>GAGAGAGAGEFMKMSGFSIEEK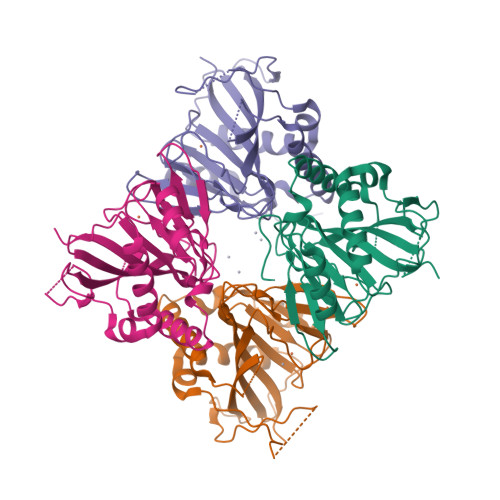VHEFESKGFLEISNEIFLQEEENHSLLTQAQLDYYNLEDDAYGECRARSYSRYIKYVDSPDYILDNSNDYFQSKEYNYDDGGKVRQFNSINDSFLCNPLIQNIVRFDTEFAFKTNIIDKSKDLIIGLHQVRYKATKERPSFSSPIWLHKDDEPVVFLHLMNLSNTAIGGDNLIANSPREINQFISLKEPLETLVFGQKVFHAVTPLGTECSTEAFRDILLVTFSYKETK[4x]> MDFQHRPGGKTGSGGVASSSESNRDRRERLRQLALETIDINKDPYFMKNHLGSY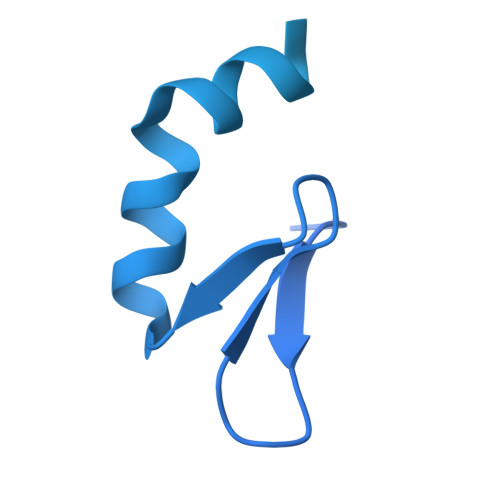ECKLCLTLHNNEGSYLAHTQGKKHQTNLARRAAKEAKEAPAQPAPEKVKVEVKKFVKIGRPGYKVTKQRDSEMGQQSLLFQIDYPEIAEGIMPRHRFMSAYEQRIEPPDRRWQYLLMAAEPYETIAFKVPSREIDKAEGKFWTHWNRETKQFFLQFHFKMEKPPAPPSLPAGPPGVKRPPPPLMNGLPPRPPLPESLPPPPPGGLPLPPMPPTGPAPSGPPGPPQLPPPAPGVHPPAPVVHPPASGVHPPAPGVHPPAPGVHPPAPGVHPPTSGVHPPAPGVHPPAPGVHPPAPGVHPPAPGVHPPAPGVHPPPSAGVHPQAPGVHPAAPAVHPQAPGVHPPAPGMHPQAPGVHPQPPGVHPSAPGVHPQPPGVHPSNPGVHPPTPMPPMLRPPLPSEGPGNIPPPPPTN> GSDLTVSLIPVSGLKAGKNAPSAKIAKLVVNSTTLKEFGVRGISNNVVDSTGTAW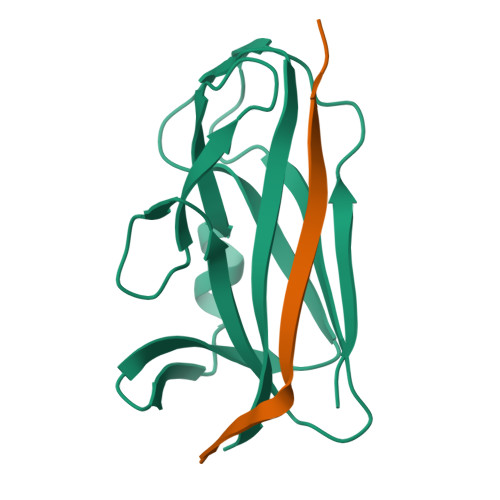RVAGKNTGKEIGVGLSSDSLRRSDSTEKWNGVNWMTFNSNDTLDIVLTGPAQNVTADTYPITLDVVGYQP;> GSFLPNSEQQKSVDIVFSSP> MKLYRLTQKKFADTPFSPIGAKLFGKRWNSKGTEALYFSESESLCSLEVFVHVNNDPAITKLYDLYRIEMPEYLIATLDEEDLPVTWRAIPASESTQYIGDQFLNDPHPEFAALQVPSTISPRDKNYVVNPNHPKMKEIIKKAEKLDFAFDPRIFK;>MATAALKSFKPKQPHKANFWFMLGIEDAETGRTDAVHKGFEPKVYRNIVERVKLSQNEFQNVTLIPVSTIKRRLKNDERFNTQESDAIYRLAMLLKLATEL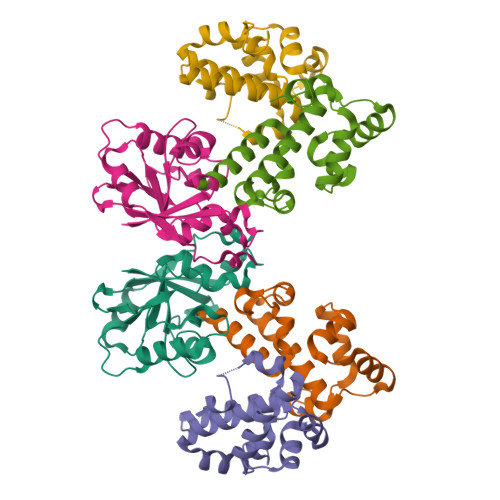FDDEERALEWMKENVYGLGGKRPLDMVSTTVDFEIVKDLIGRLEHGVFS[2x]> AQAGHYITKNGNDWQYDTNGELAKGLRQDSNGKLRYFDLTTGIQAKGQFVTIGQETYYFSKDHGDAQLLPMVTEGHYGTITLKQGQDTKTAWVYRDQNNTILKGLQNINGTLQFFDPYTGEQLKGGVAKYDDKLFYFESGKGNLVSTVAGDYQDGHYISQDGQTRYADKQNQLVKGLVTVNGALQYFDNATGNQIKNQQVIVDGKTYYFDDKGNGEYLFTNTLDMSTNAFSTKNVAFNHDSSSFDHTVDGFLTADTWYRPKSILANGTTWRDSTDKDMRPLITVWWPNKNVQVNYLNFMKANGLLTTAAQYTLHSDQYDLNQAAQDVQVAIERRIASEHGTDWLQKLLFESQNNNPSFVKQQFIWNKDSEYHGGGDAWFQGGYLKYGNNPLTPTTNSDYRQPGNAFDFLLANDVDNSNPVVQAENLNWLHYLMNFGTITAGQDDANFDSIRIDAVDFIHNDTIQRTYDYLRDAYQVQQSEAKANQHISLVEAGLDAGTSTIHNDALIESNLREAATLSLTNEPGKNKPLTNMLQDVDGGTLITDHTQNSTENQATPNYSIIHAHDKGVQEKVGAAITDATGADWTNFTDEQLKAGLELFYKDQRATNKKYNSYNIPSIYALMLTNKDTVPRMYYGDMYQDDGQYMANKSIYYDALVSLMTARKSYVSGGQTMSVDNHGLLKSVRFGKDAMTANDLGTSATRTEGLGVIIGNDPKLQLNDSDKVTLDMGAAHKNQKYRAVILTTRDGLATFNSDQAPTAWTNDQGTLTFSNQEINGQDNTQIRGVANPQVSGYLAVWVPVGASDNQDARTAATTTENHDGKVLHSNAALDSNLIYEGFSNFQPKATTHDELTNVVIAKNADVFNNWGITSFEMAPQYRSSGDHTFLDSTIDNGYAFTDRYDLGFNTPTKYGTDGDLRATIQALHHANMQVMADVVDNQVYNLPGKEVVSATRAGVYGNDDATGFGTQLYVTNSVGGGQYQEKYAGQ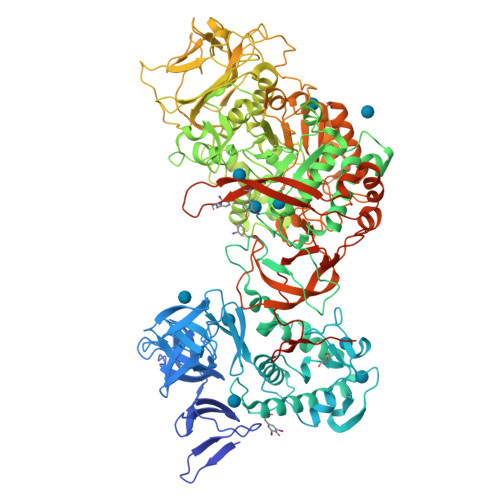YLEALKAKYPDLFEGKAYDYWYKNYANDGSNPYYTLSHGDRESIPADVAIKQWSAKYMNGTNVLGNGMGYVLKDWHNGQYFKLDGDKSTLPQIKGELKLEGKPIPNPLLGLDSTRTGHHHHHH> MDDFASLPLVIEPADLQARLSAPELILVDLTSAARYAEGH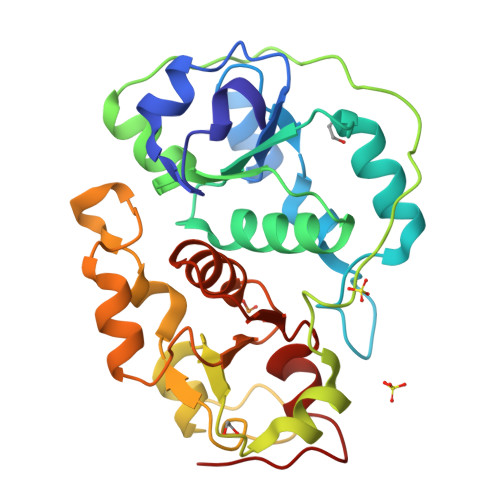IPGARFVDPKRTQLGQPPAPGLQPPREQLESLFGELGHRPEAVYVVYDDEGGGWAGRFIWLLDVIGQQRYHYLNGGLTAWLAEDRPLSRELPAPAGGPVALSLHDEPTASRDYLLGRLGAADLAIWDARSPQEYRGEKVLAAKGGHIPGAVNFEWTAAMDPSRALRIRTDIAGRLEELGITPDKEIVTHCQTHHRSGLTYLIAKALGYPRVKGYAGSWGEWGNHPDTPVEL>GTSQLAELVDAAAERLEVADPVAAFKWRAQLPIEDSGRVEQQLAKLGEDARSQHIDPDYVTRVFDDQIRATEAIEYSRFSDWKLNPASAP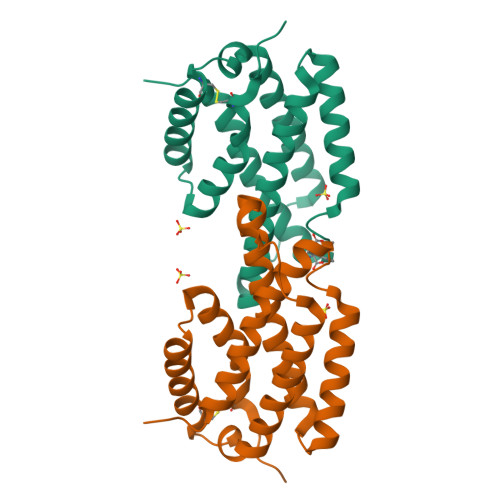PEPPDLSASRSAIDSLNNRMLSQIWSHWSLLSAPSCAAQLDRAKRDIVRSRHLDSLYQRALTTATQSYCQALPPA[3x]(2R)-2-ETHYL-1-HEXANESULFONIC 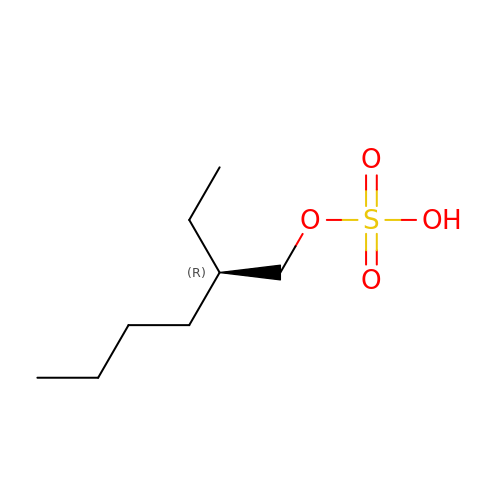ACID | C8 H18 O4 S | MHGOKSLTIUHUBF-MRVPVSSYSA-N>MPNIKIFSGSSHQDLSQKIADRLGLELGKVVTKKFSNQETCVEIGESVRGEDVYIVQSGCGEINDNLMELLIMINACKIASASRVTAVIPCFPYARQDKKDKSRAPISAKLVANTLSVAGADHIITMDLHASQIQGFFDIPVDNLYAEPAVLKWIRENISEWRNCTIVSPDAGGAKRVTSIADR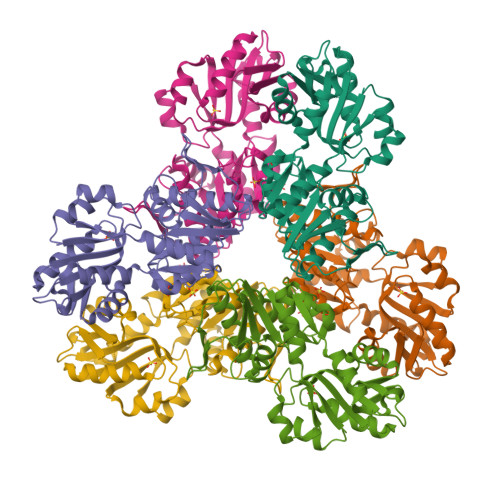LNVDFALIHKERKKANEVDRMVLVGDVKDRVAILVDDMADTCGTICHAADKLLSAGATRVYAILTHGIFSGPAISRINNACFEAVVVTNTIPQEDKMKHCSKIQVIDISMILAEAIRRTHNGESVSYLFSHVPLLEHHHHHH[2x]>MGSHHHHHHASEQYPTAIVADREVPFDPEQLRRIREHPCFSEKACHAFGRMHLPVAPKCNIQCKYCIRDFDCVNESRPGVTSRVLTPQEALERVDEVLSKYHYIKVVAVAGPGEPLANEETFETLRLVGEKYPHLILCISTNGLLLPDRIEDLDRIGVTNITVTLNAVDPTIGEQIYDYVIYKGERYEGLEAAKILLDNQLKGIEEAVRRKKIVKVNTVLIPGINDKHVFDIARKIKSMGVFIHNVMPLIPQYKFAHIKPPTPEEKRAIQDELSKIIKQMRHCRQCRSDAIGRLGCDIQQELEK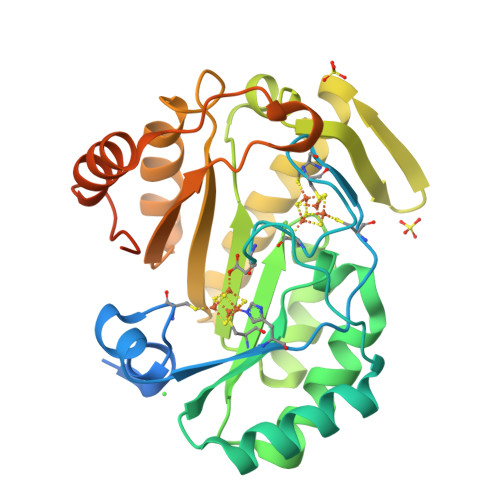GKKKS[2x]>MLQSQFAQTPRLALADTVIDLKARKNLSWQALTDGTGLSLAFVTAALLGQHPLPKEAADI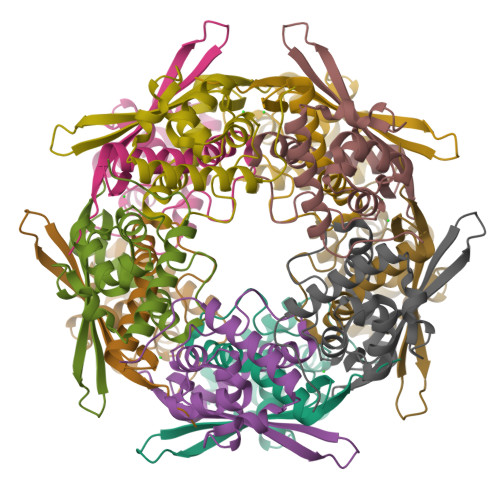VCGKLGLDEDASRLLQSVPLRGSFPSGVPTDPTMYRFYEMLQVYGSTLKALVHEQFGDGIISAINFKLDIKKVEDPDGGSRAVITLDGKYLPTKPF[10x]>[60x]GSGVGISTGGWVGGSHFSDKYVVTKNTRQFITTIQNGHLYKTEAIETTNQSGKSQRCVTTPWTYFNFNQYSCHFSPQDWQRLTNEYKRFRPKAMQVK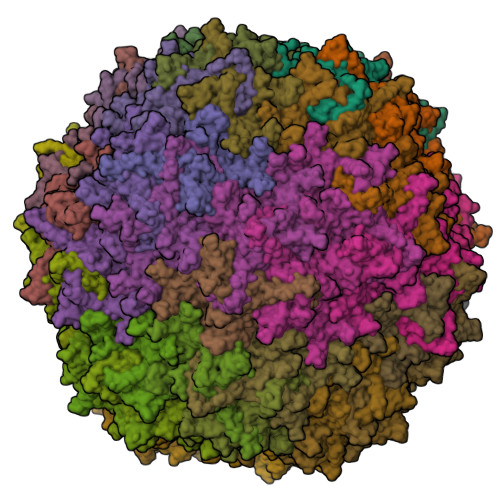IYNLQIKQILSNGADTTYNNDLTAGVHIFCDGEHAYPNASHPWDEDVMPDLPYKTWKLFQYGYIPIENELADLDGNAAGGNATEKALLYQMPFFLLENSDHQVLRTGESTEFTFNFDCEWVNNERAYIPPGLMFNPKVPTRRVQYIRQNGSTAASTGRIQPYSKPTSWMTGPGLLSAQRVGPQSSDTAPFMVCTNPEGTHINTGAAGFGSGFDPPSGCLAPTNLEYKLQWYQTPEGTGNNGNIIANPSLSMLRDQLLYKGNQTTYNLVGDIWMFPNQVWDRFPITRENPIWCKKPRADKHTIMDPFDGSIAMDHPPGTIFIKMAKIPVPTASNADSYLNIYCTGQVSCEIVWEVERYATKNWRPERRHTALGMSLGGESNYTPTYHVDPTGAYIQPTSYDQCMPVKTNINKVL> SNFADSFNIKTFEKWVTVAEASIIRQKTDTDETIDCMNRFIKMLESTMNGISHFPLKTFKSGSYYDRTKIDYNDEFDFMFFPDMKMEAVFTNCPPGYCKIRKGVTNSKDLDPYLNKDGFLVPGLFKQAMFDLFEKSLSDGTFREGRRTTRQTSKPGSPAYTILYNLGIHGKRPIDVDLVPAIRIECWPKPAKEIKPDWVKKETTERATRCFHAVMKTYPENWPDGDLLWRISFTHAEKELILHANEKEKGCRKDIFRLLKKIKEVMKSRNSNDIDKFCSYHLKMFML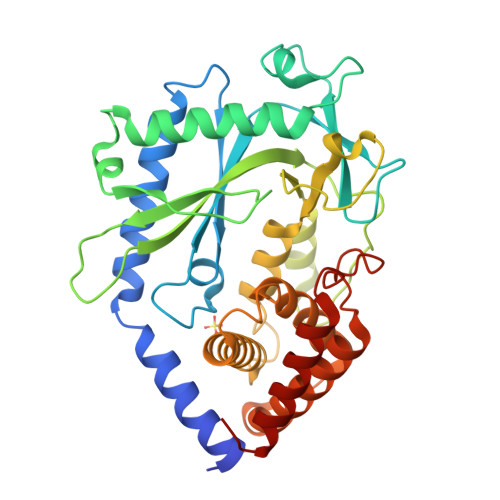KFFDKEKYFRNEMKVDLLKKAIKKLGESVEHGNIPNYFIPEDNVIVNVLEKERTLIAKELRALLEGNW> SGFNNDPFVQRKLGTSGLNQPTFQQTDLSQVWPEANQHFSKEIDDEANSYFQRIYNHPPHPTMSVDEVLEMLQRFKDSTIKREREVFNCMLRNLFEEYRFFPQYPDKELHITACLFGGIIEKGLVTYMALGLALRYVLEALRKPFGSKMYYFG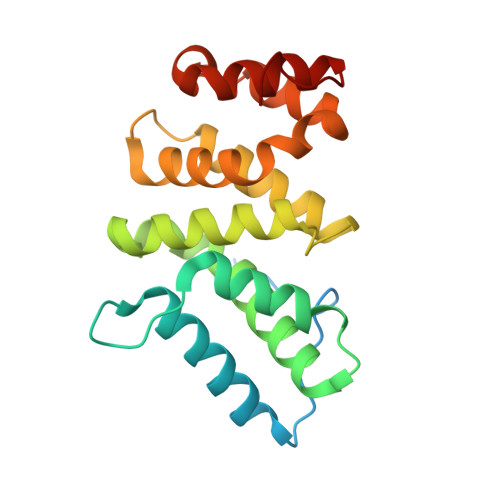IAALDRFKNRLKDYPQYCQHLASISHFMQFPHHLQEYIEYGQQSRDPPVK>MDFTKPETVLNLQNIRDELVRMEDSIIFKFIERSHFATCPSVYEANHPGLEIPNFKGSFLDWALSNLEIAHSRIRRFESPDETPFFPDKIQKSFLPSINYPQILAPYAPEVNYN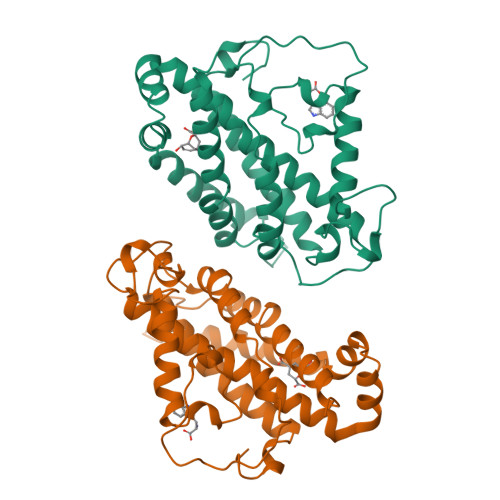DKIKKVYIEKIIPLISKRDGDDKNNFGSVATRDIECLQSLSRRIHFGKFVAEAKFQSDIPLYTKLIKSKDVEGIMKNITNSAVEEKILERLTKKAEVYGVDPTERRIERRITPEYLVKIYKEIVIPITKEVEVEYLLRRLEE[2x]>SRPQSTLRRAITAAYRRPETECLPPLVEAATQSKEIRDAAASTARKLIEALRGKHSGSGSSGSMMGEQFVTGETIREALKRSKELEEKGFSYSYDMLGEAATTAADAERYYRDYESAIHAIGKASAGRGIYEGPGISIKLSALHPRYSRAQAARVMGELLPRVKALALLAKNYDIGLNIDAEEADRLELSLDLLEVLCLDGDLSGWNGMGFVVQAYGKRCPFVLDFIIDLARRSGRRIMVRLVKGAYWDAEIKRAQLDGLADFPVFTRKIHTDVSYIACAAKLLAATDVVFPQFATHNAQTLAAIYHMAGKDFHVGKYEFQCLHGMGEPLYEEVVGRGKLDRPCRIYAPVGTHETLLAYLVRRLLENGANSSFVHRINDPKV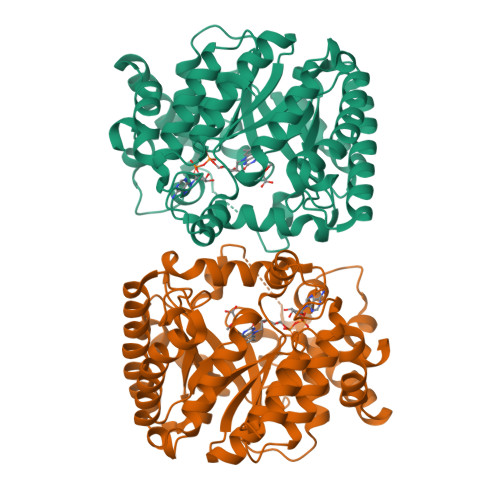SIDELIADPVEVVR[2x]3-chloro-4-({(2S)-2-[2-(4-chlorophenyl)-5,6-difluoro-1H-benzimidazol-1-yl]-2-cyclohexylacetyl}amino)benzoic acid | C28 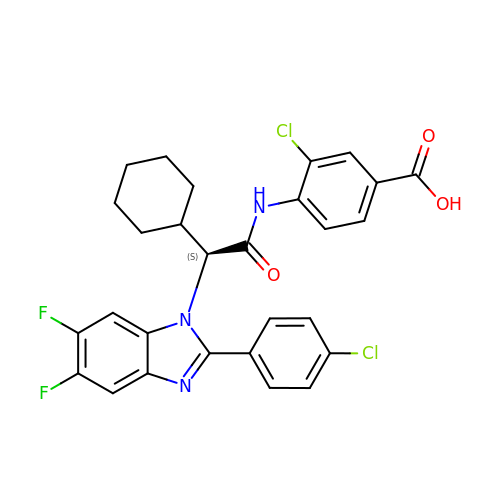H23 Cl2 F2 N3 O3 | OLLRSJLKNAIFCJ-VWLOTQADSA-N>MIFEVLKILTDEVNQNFKGLEMEDSEVVLNNVALIDSQQDVATELQNKVILSMINLREEVTMKNFPNNVLEGTKVTYKNPKLNINLFLI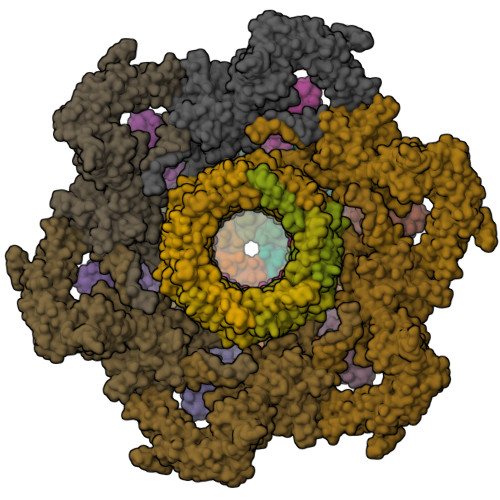FCANRTGYKKSLSDLSRILEFFQHKSVFTQSNTSFDRDLEEMENVKNFRFTMELFTPTFEELNYIWGTLGGRQYPSVFYKLNLIVIDRDATTSEEGVITNIHRNYETL[6x];>[6x]MQVSSSFRSFLKLDILHSYFLNDGEKDFSSMNEEESKTQLKSYNWKDFLEIYPSQKTSHMMRGNKIFFKSFNDSIILAIKVESGTENQPFNELYEDESMTFLLSLKDQYFGNYTDLDLADQLLYFSNKTPVLPEAFTFKPIDRINQSGTVGEEYLYEGENKKHLLEEAHLNPGGGVLGIIQIYMKGDTPVLSLINNDGTLKNSLPHFKIHFSNRKSTWKYINLKDDFETETKKDYPLTKFGFILLDKKSDFISPPAHFEKYVFPNPDARRIKITPTKNYSEIFI;>MSYPLSKFHFSVEWGGTKIGFTEVSGLDLETEIIEYRHGASPEYSKIKMPGMQKFSNITLKRGTFKSDNEYFQWYNTINLNKVERRDLTISLLNEEHEPVVTWKVKNAWPLKVQSTDLKGDGNEVAIESMELAHEGLVIQNE[12x];>[6x]MATYKTPGVYIEEITKFPPSVAQVETAIPAFIGYTQFARTKPSVDSDDLILKPKRISSLLDFTTYYGGAQNEQGITVKLTDTLIEGAENRTINVPEPTFKSPYLMFYSLQMYFANGGGPCYIVSTGVYDDWSDSETPPTINFSDLESGLAVIRKEDEPTLLLFPDATNLPTDDEFYSLYNSALMQCNDLQDRFTILDTYSDQTYNDGVEDLDPIPALRNGINLTKDYLKYGAAYYPFVQTILNYQYSADEIVIQHLSYNPNAIATALDNLNAVNGPTFIDAILDDLRDLSLPDISGEISDAVGFMYDDVDGFDIDGTFTTNSVKVANFASLVESVLSTLNELIDAKEEINKDVNSAIASSEEDNAIKTAISDALDVFNEDFEGADKIESVAKNLSDLLIKIKQADTNTKVENVLSINALNFSAEFEKLLTYDVNTGLTASVTLDLFANIGTRLDDIIAAVSAAEPIDVNNGKLNGRLLSDIEPLDNATYNTILLEINSHKVTLPPSSSMAGAYARVDNDRGVWKSPANIGLNYVSKPSVTVSHEEQESMNVHGTGKSVNAIRSFVGKGTLVWGARTLAGNDNEWRYISVRRFFNMAEESIKKATEQFVFEPNDGNTWVRVRAMIENFLILQWRAGALAGAKPEHAFYVKVGLGQTMTAQDILEGNMNVEIGLAVVRPAEFIILKFSHKMQES> MGSSHHHHHHSSGLVPRGSHMSPSPVPGSQNVPAPAVKKISQYACQRRTTLNNYNQLFTDALDILAENDELRENEGSCLAFMRASSVLKSLPFPITSMKDTEGIPCLGDKVKSIIEGIIEDGESSEAKAVLNDERYKSFKLFTSVFGVGLKTAEKWFRMGFRTLSKIQSDKSLRFTQMQKAGFLYYEDLVSCVNRPEAEAVSMLVKEAVVTFLPDALVTMTGGFRRGKMTGHDVDFLITSPEATEDEEQQLLHKVTDFWKQQGLLLYHQYHRSHLADSAHNLRQRSSTMDVFERSFCILKLDHGRVHSEKSGQQEGKGWKAIRVDLVMCPYDRRAFALLGWTGSRQFERDLRRYATHERKMMLDNHALYDRTKRVFLEAESEEEIFAH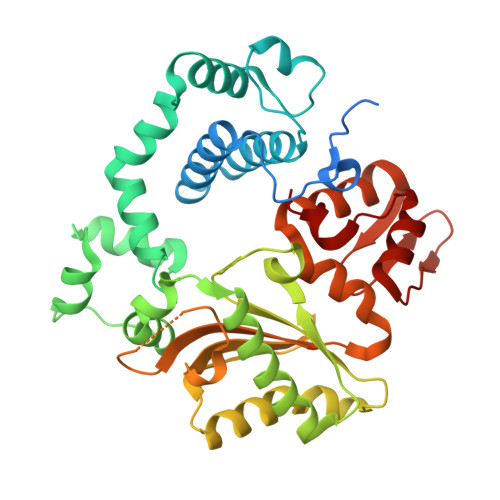LGLDYIEPWERNA>MALADISGYLDVLDSVRGFSYLENAREVLRSGEARCLGNPRSEPEYVKALYVIGASRIPVGDGCSHTLEELGVFDISVPGEMVFPSPLDFFERGKPTPLVRSRLQLPNGVRVWLKLEWYNPFSLSVADRPAVEIISRLSRRVEKGSLVADATSSNFGVALSAVARLYGYRARVYLPGAAEEFGKLLPRLLGAQVIVDPEAPSTVHLLPRVMKDSKNEGFVHVNQFYNDANFEAHMRGTAREIFVQSRRGGLALRGVAGSLGTSGHMSAAAFYLQSVDPSIRAVLVQPAQGDSIPGIRRVETGMLWINMLDISYTLAEVTLEE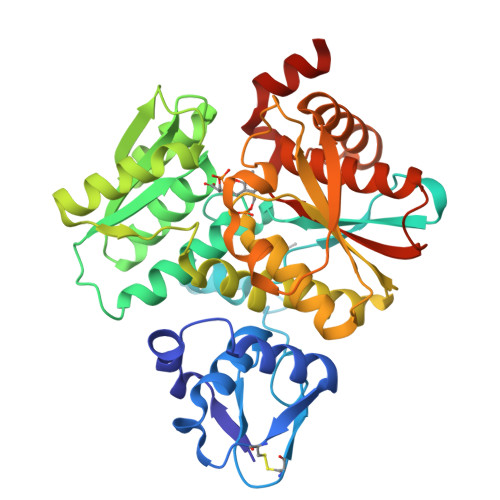AMEAVVEVARSDGLVIGPSGGAAVKALAKKAAEGDLEPGDYVVVVPDTGFKYLSLVQNALEGAGDSV[2x]> STAGKVIKCKAAVLWEEKKPFSIEEVEVAPPKAHEVRIKMVATGICRSDDHVVSGTLVTPLPVIAGHEAAGIVESIGEGVTTVRPGDKVIPLFTPQCGKCRVCKHPEGNFCLKNDLSMPRGTMQDGTSRFTCRGKPIHHFLGTSTFSQYTVVDEISVAKIDAASPLEKVCLIGCGFSTGYGSAVKVAKVTQGSTCAVFGLGGVGLSVIMGCKAAGAARIIGVDINKDKFAKAKEVGATECVNPQDYKKPIQEVLTEMSNGGVDFSFEVIGRLDTMVTALSCCQEAYGVSVIVGVPPDSQNLSMNPMLLLSGRTWKGAIFGGFKSKDSVPKLVADFMAKKFALDPLIT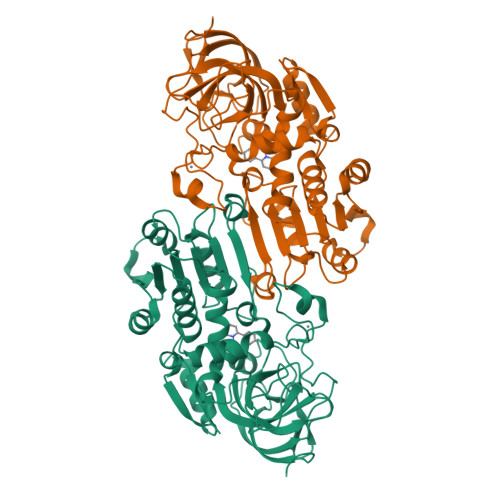HVLPFEKINEGFDLLRSGESIRTILTF 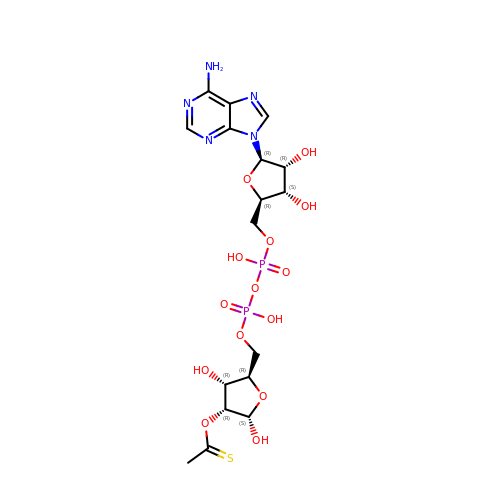thioacetyl-ADP-ribose | C17 H25 N5 O14 P2 S | KCGNVGFYYIVLLI-DLFWLGJNSA-N> MTVKVCVCGGGNGAH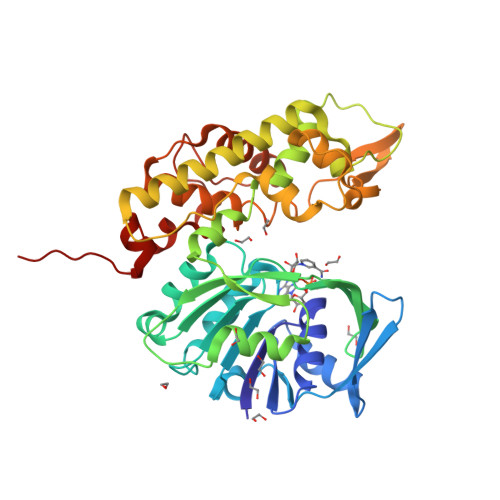TLSGLAASRDGVEVRVLTLFADEAERWTKALGADELTVIVNEKDGTQTEVKSRPKVITKDPEIAISGADVVILTVPAFAHEGYFQAMAPYVQDSALIVGLPSQAGFEFQCRDILGDKAAAVSMMSFETLPWACRIKEFGRKVEVLGTKSVLAASLIKGTAKTVDPLSTLQMLHGAEPVFRLAKHFLEMLIMSYSFVHPAILFGRWGSWDGKPVPEAPLFYQGIDQATADMLTACSNECKDVANAIMAACPGNDLSDVKDIYQWYLEYYHEDIQDDHDLYHAITTNKSYKGLVHPVKAVDGGVAPDFGNRYLTEDIPMGMIVFKGVAIAAGVAIPSNDKLIMWAQEKIGKEYLVDGALTGKDVATTRCPQRYGFNTLDAILTGKKHHHHH> MGTVSSRRSWWPLPLLLL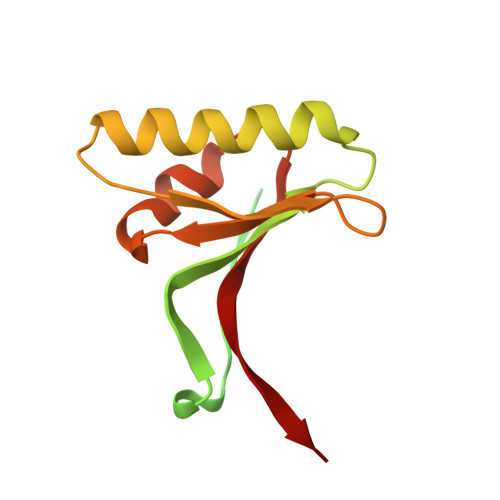LLLLLGPAGARAQEDEDGDYEELVLALRSEEDGLAEAPEHGTTATFHRCAKDPWRLPGTYVVVLKEETHLSQSERTARRLQAQAARRGYLTKILHVFHGLLPGFLVKMSGDLLELALKLPHVDYIEEDSSVFAQ>[2x]MAETVESLAKSHIEGSFTNVWKDDKTLDWYANYEGILWKATGVVVITGDETQVYAIWVP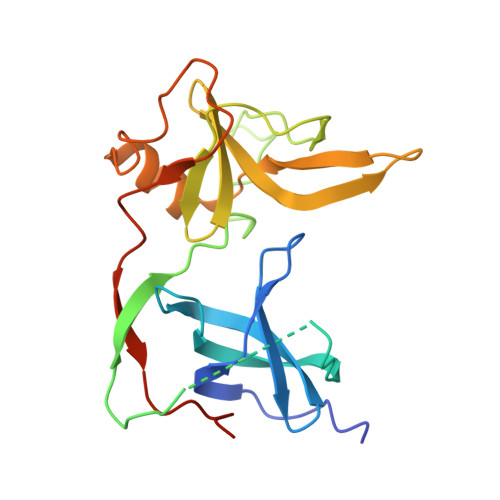VGLAIPENEGGGSEGGGSEGGGSEGGGTKPPEYGDTPIPGYIYINPLDGTYPPGTEQNPANPNPSLEESHPLNTFMFQGNRFRNVNGVLTVYTGTVTVNGKTYYQYTPVSSKAMYDAYWNGKFRDVAFHSGFNEDPLVAEYQGQLSYLPQPPVNAPSGHHHHHH> GAMAFD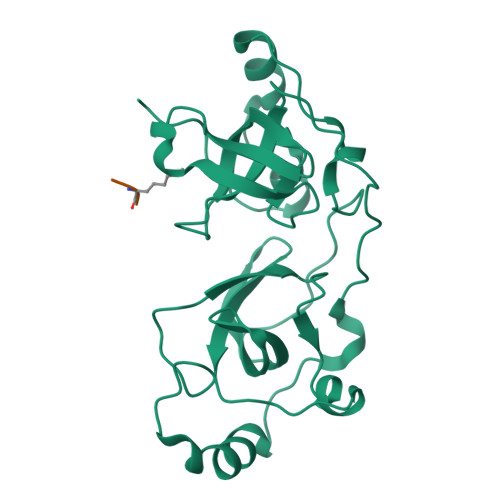WDAYLEETGSEAAPAKCFKQAQNPPNNDFKIGMKLEALDPRNVTSTCIATVVGVLGSRLRLRLDGSDSQNDFWRLVDSTEIHAIGHCEKNGGMLQPPLGFCMNASSWPGYLCKILNNAMVAPEEIFQPEPPEPEENLFKVGQKLEAVDKKNPQLICCATVDAIKDDQIHVTFDGWRGAFDYWCNYRSRDIFPAGWCARSCHPMQPPGHKSRMDSSSSKQRCPRPRYTVVAESEAMVPASPATAHFHPNCKGGPFINNSK;> RKS Tripartite motif-containing protein (TRIM)72 (mitsugumin 53; MG53) has been determined to rapidly nucleate vesicles at the site of membrane damage, but the underlying molecular mechanisms remain poorly understood. Here we present the structure of Mus musculus TRIM72, a complete model of a TRIM E3 ubiquitin ligase. TRIM72 is a member of the class IV TRIM proteins, which is the largest subtype among the 11 groups of TRIM proteins. Its domain organization includes an RBCC domain followed by a PRY motif associated with a SPRY domain identified in splA kinase and ryanodine receptors (PRYSPRY) domain.

The coiled-coil domains (CCDs) form the main scaffold of an antiparallel dimer with a length of approximately 17 nm. In the middle of the CCDs, the structural core consists of the hendecad repeated region of the H1:H1′ helices (prime indicates the second protomer of the dimer) and the H3:H3′ helices followed by a pair of PRYSPRY domains. Between the H1:H1′ helices and PRYSPRY domains, the H3:H3′ helices are sandwiched to interact with both domains. Owing to these interdomain interactions, two PRYSPRY domains are located on the opposite side of the CCDs across the H3:H3′ helices. Recent cryo-electron microscopy (EM) analysis of TRIM72 and the crystal structure of TRIM72 ΔRING also revealed that the CCD ends are dynamic. These results suggest that the flexibility of long TRIM CCDs is suitable for recognizing curved cellular structures, such as phospholipid membranes and viral capsids, and filamentous structures, such as dsRNA and DNA.

>[2x]GSAQVPQGHCEEHLDPLSIYCEQDRTLVCGVCASLGSHRGHRLLPAAEAQARLKTQLPQQKMQLQEASMRKEKTVAVLEHQLVEVEETVRQFRGAVGEQLGKMRMFLAALESSLDREAERVRGDAGVALRRELSSLNSYLEQLRQMEKVLEEVADKPQTEFLMKFSLVTSRLQKILSESPPPARLDIQLPVISDDFKFQVWKHMFRHLMPALEELTFDPSSAHPSLVVSSSGRRVECSDQKAPPAGEDTRQFDKAVAVVAQQLLSQGEHYWEVEVGDKPRWALGVMAADASRRGRLHAVPSQGLWLLGLRDGKILEAHVEAKEPRALRTPERPPARIGLYLSFADGVLAFYDASNPDVLTPIFSFHERLPGPVYPIFDVCWHDKGKNAQPLLLV>RPQGATVSLWETVQKWREYRRQCQRSLTEDPPPATDLFCNRTFDEYACWPDGEPGSFVNVSCPWYLPWASSVPQGHVYRFCTAEGLWLQKDNSSLPWR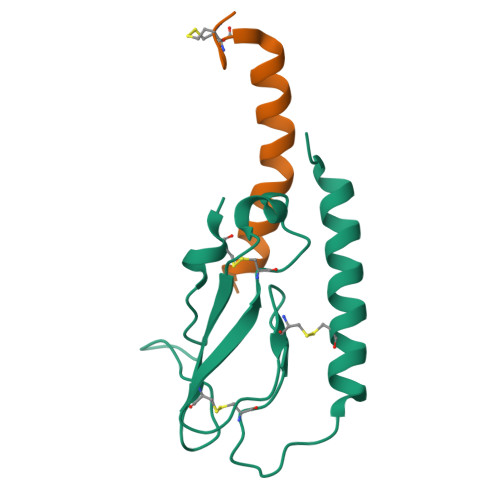DLSECEESKRGERSSPEE[2x];>HXEGXFTSDVSSYLEGQAAKEFIAWLVKGRG[2x]> MKHHHHHHPMAVTIDYWDTITIKHKETKAYLHSHPDRYPLRYDDGRVSSQGQQVTGYPFNDTNNWWQILPAGPFEEPKLGRHVKHRDLVRLRHVGTDTYLLSHDVASPYYPTNQEFTTVSFNEAYGDRAADTLFEVRIEHGKPGQEFKSISSHFKLIHNPSKVAMWTHPTPLPDWGHRQQEINGNKQIAPSSNVWLVEDIVSLPADHKRRE

Protein O-mannosyltransferases (PMTs) are conserved endoplasmic reticulum membrane-embedded enzymes responsible for the transfer of mannose from dolichol phosphate-mannose (Dol-P-Man) to serine/threonine-rich protein substrates or unfolded proteins. PMTs from three subfamilies form obligate dimers with different substrate specificities and require the concerted action of their transmembrane domains (TMDs) and a luminal MIR domain for catalysis. Here, we present structures, native mass spectrometry, and structure-based mutagenesis of the fungal Pmt4 homodimer. The core fold of the TMDs and MIR domain is conserved with the Pmt1-Pmt2 heterodimer, indicating a shared catalytic mechanism.

Therefore, we purified the ctPmt4-MIR domain from Escherichia coli via a N-terminal hexa-histidine tag and solved the crystal structure at 1.2 Å resolution by molecular replacement. Therefore, in order to be able to compare PMT2 and PMT4 family MIR domains from the same species, we additionally purified the scPmt4-MIR domain and solved the crystal structure to 1.3 Å resolution. Aside from minor conformational differences in the β4−β5 and β8−β9 loops, the scPmt4- and ctPmt4-MIR domain structures are highly similar (RMSD 0.87 Å over 194 Cα-atoms) and comprise the characteristic peculiar β-trefoil fold i.e. six β-hairpins arranged within a pseudo-threefold symmetry (three MIR-motifs: MIRm1,2,3), altogether forming a β-barrel and a triangular cap. Characteristically, the Pmt4-MIR domain structures reveal a unique β-hairpin insertion (β-ins) of seven residues (RY(D/E)(D/N)GRΦ) in β2−β3 of MIRm1. β-ins is extensively stabilised by internal hydrogen-bonding and a central salt-bridge between the conserved 4th and 6th residue (ct: D370:R372, sc: D364:R366). It is fixed on top of the cap scaffold by hydrogen-bonding of the tyrosine (ct: Y368, sc: Y362) to a glutamate (ct: E441, sc: E434), and of the centrally-fixed arginine to the mainchain around a proline (ct: P434, sc: P427) within MIRm2. As observed previously in the PMT2-MIR crystal structures, the Pmt4-MIR domains are extensively bound to small polar ligands present in the crystallisation solutions (acetate or HEPES) or cryo-protectant buffers (glycerol or ethylene glycol). In particular, the α and β sites, which were demonstrated for scPmt2 to bind O-mannosylated peptides, are again occupied by ligands in ctPmt4-MIR and scPmt4-MIR respectively, in-line with the expectation that they are also sugar binding sites. Given that both the open γ site and β-ins of ctPmt4-MIR are also bound to acetate ligands, these too may be mannose binding sites, which would indeed provide an explanation for the importance of β-ins in O-mannosylation by Pmt4. Furthermore, the ctPmt4- and scPmt4-MIR domains have an asymmetric surface charge distribution with both a highly positively and negatively charged patch.> MKKFASLILTSVFLFSSTQFVHASSTDVQERLRDLAREDEAGTFNEAWNTNFKPSDEQQFSYSPTEGIVFLTPPKNVIGERRISQYKVNNAWATLEGSPTEASGTPLYAGKNVLDNSKGTMDQELLTPEFNYTYTESTSNTTTHGLKLGVKTTATMKFPIAQGSMEASTEYNFQNSSTDTKTKQVSYKSPSQKIKVPAGKTYRVLAYLNTGSISGEANLYANVGGIAWRVSPGYPNGGGV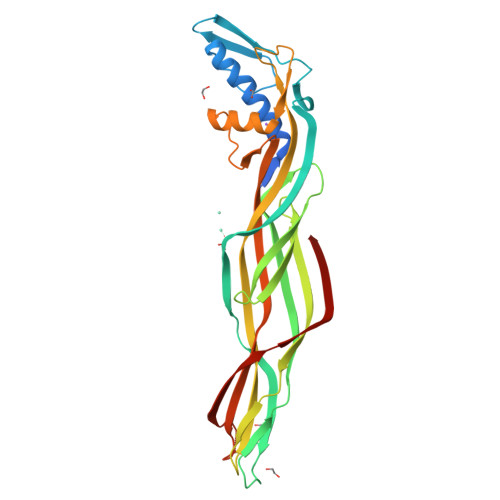NIGAVLTKCQQKGWGDFRNFQPSGRDVIVKGQGTFKSNYGTDFILKIEDITDSKLRNNNGSGTVVQEIKVPLIRTEIHHHHAHHH> MSQSQEAKNALIIAQLKGDFVAFLFVLWKALNLPKPTKCQIDMARTLANGDHKKFILQAFRGIGKSFITCAFVVWVLWRDPQLKVLIV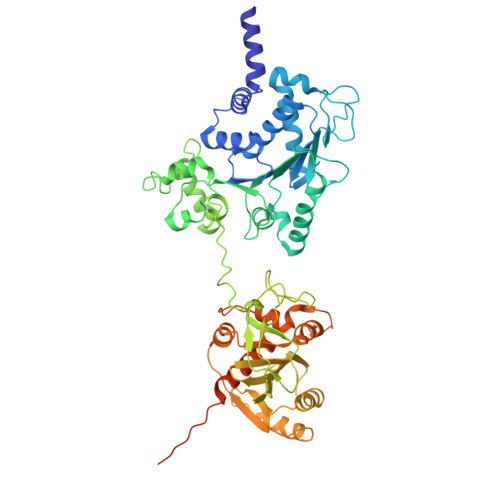SASKERADANSIFIKNIIDLLPFLSELKPRPGQRDSVISFDVGLAKPDHSPSVKSVGITGQLTGSRADIIIADDVEVPGNSSTSSAREKLWTLVTEFAALLKPLPTSRVIYLGTPQTEMTLYKELEDNKGYSTVIWPAQYPRNDAEALYYGDRLAPMLKAEYDEGFELLRGQPTDPVRFDMDDLRERELEYGKAGYTLQFMLNPNLSDAEKYPLRLRDAIVCAVDPERAPLSYQWLPNRQNRNEELPNVGLKGDDIHAFHTCSSRTAEYQSKILVIDPSGRGKDETGYAVLYSLNGYIYLMEVGGFRGGYDDATLEKLAKKAKQWKVQTVVHESNFGDGMFGKIFSPILLKHHKCALEEIRAKGMKEMRICDTIEPLMGAHKLVIRDEVIREDYQTARDLDGKHDVRYSAFYQMTRMTRERGAVAHDDRIDAIALGIEYLREGMLVDSRVGEEEMTLEFLEHHMEKQTIGGDQIHSFDVGGVDIYYEDEDGGSSFIEW>[4x]KFSAKRLPSTRLGTFLENRVNDFLRRQNHPESGEVTVRVVHASDKTVEVKPGMKARFVDSGEMAESFPYRTKALFAFEEIDGVDLCFFGMHVQEYGSDCPPPNQRRVYISYLDSVHFFRPKCLRTAVYHEILIGYLEYVKKLGYTTGHIWACPPSEGDDYIFHCHPPDQKIPKPKRLQEWYKKMLDKAVSERIVHDYKDI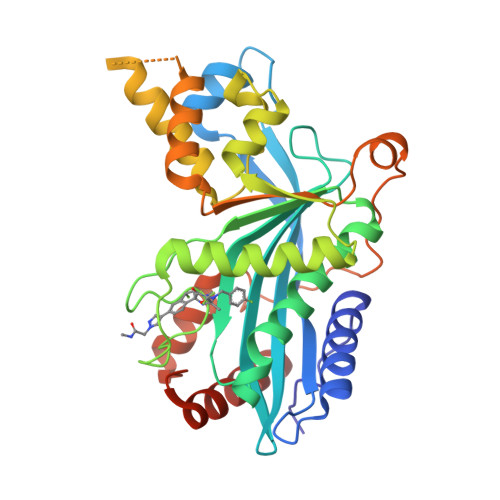FKQATEDRLTSAKELPYFEGDFWPNVLEESIKELEQKTSKNKSSLSRGNKKKPGMPNVSNDLSQKLYATMEKHKEVFFVIRLIAGPAANSLPPIVDPDPLIPCDLMDGRDAFLTLARDRHLEFSSLRRAQWSTGCMLVELHTQSQDRF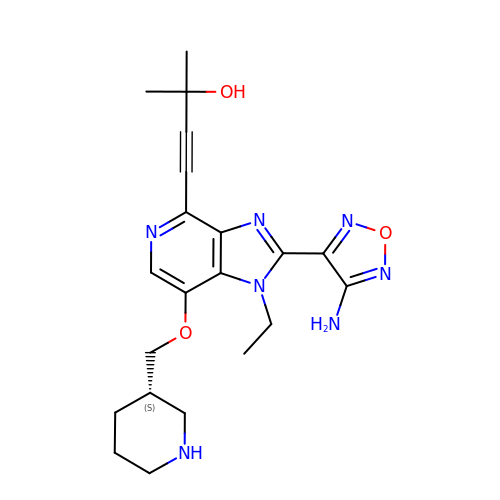4-{2-(4-amino-1,2,5-oxadiazol-3-yl)-1-ethyl-7-[(3S)-piperidin-3-ylmethoxy]-1H-imidazo[4,5-c]pyridin-4-yl}-2-methylbut-3-yn-2-ol | C21 H27 N7 O3 | KGPGFQWBCSZGEL-ZDUSSCGKSA-N>[5x]MTQELGNANFENFIGATEGFSEIAYQFTSHILTLGYAVMLAGLLYFILTIKNVDKKFQMSNILSAVVMVSAFLLLYAQAQNWTSSFTFNEEVGRYFLDPSGDLFNNGYRYLNWLIDVPMLLFQILFVVS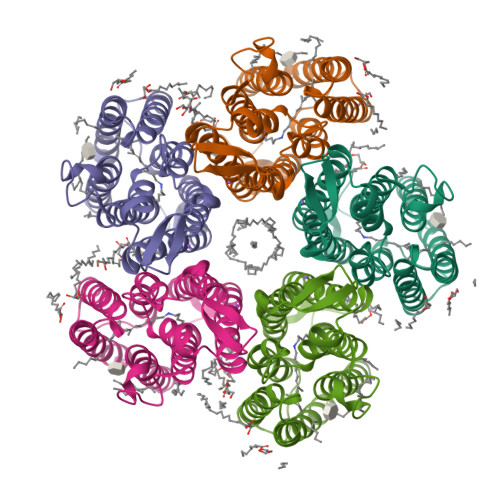LTTSKFSSVRNQFWFSGAMMIITGYIGQFYEVSNLTAFLVWGAISSAFFFHILWVMKKVINEGKEGISPAGQKILSNIWILFLISWTLYPGAYLMPYLTGVDGFLYSEDGVMARQLVYTIADVSSKVIYGVLLGNLAITLSKNKELVEANSLEHHHHHH>[2x]HMSKAFDLVVIGAGSGGLEAGWNAATLYGKRVAVVDVQTSHGP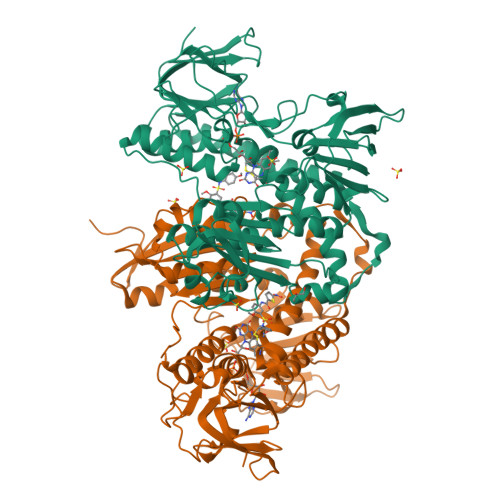PFYAALGGTCVNVGCVPKKLMVTGAQYMDHLRESAGFGWEFDGSSVKANWKKLIAAKNEAVLDINKSYEGMFNDTEGLDFFLGWGSLESKNVVVVRETADPKSAVKERLQADHILLATGSWPQMPAIPGIEHCISSNEAFYLPEPPRRVLTVGGGFISVEFAGIFNAYKPPGGKVTLCYRNNLILRGFDETIREEVTKQLTANGIEIMTNENPAKVSLNTDGSKHVTFESGKTLDVDVVMMAIGRIPRTNDLQLGNVGVKLTPKGGVQVDEFSRTNVPNIYAIGDITDRLMLTPVAINEGAALVDTVFGNKPRKTDHTRVASAVFSIPPIGTCGLIEEVAAKEFEKVAVYMSSFTPLMHNISGSKYKKFVAKIVTNHSDGTVLGVHLLGDGAPEIIQAVGVCLRLNAKISDFYNTIGVHPTSAEELCSMRTPSYYYVKGEKMEKLPDSNL>[6x]NLDNKLDGFYIAPAFMDKLVVHITKNFLKLPNIKVPLILGIWGGKGQGKSFQCELVFRKMGINPIMMSAGELESGNAGEPAKLIRQRYREAAEIIRKGNMCCLFINDL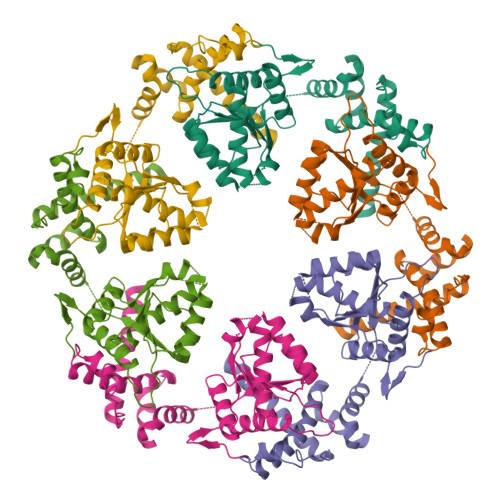DAGAGRMGGTTQYTVNNQMVNATLMNIADNPTNVQLPGMYNKQENARVPIIVTGNDFSTLYAPLIRDGRMEKFYWAPTREDRIGVCTGIFRTDNVPAEDVVKIVDNFPGQSIDFFGALRARVYDDEVRKWVSGTGIEKIGDKLLNSFDGPPTFEQPKMTIEKLLEYGNMLVQEQENVKRVQLADK>[2x]MHHHHHHQIGWRREGIKYRRNELFLDVLESVNLLMSPQGQVLSAHVSGRVVMKSYLSGMPECKFGMNDKIVIEKQGKGTADETSKSGKQSIAIDDCTFHQCVRLSKFDSERSISFIPPDGEFELMRYRTTKDIILPFRVIPLVREVGRTKLEVKVVIKSNFKPSLLAQKIEVRIPTPLNTSGVQVICMKGKAKYKASENAIVWKIKRMAGMKESQISAEIELLPTNDKKKWARPPISMNFEVPFAPSGLKVRYLKVFEPKLNYSDHDVIKWVRYIGRSGIYETRC;>SDLLAWDPLFG[2x]

Proper operation of the pivotal CME cargo adaptor AP2 requires membrane-localized Fer/Cip4 homology domain-only proteins (FCHO). The AP2 complex, composed of α, β2, μ2, and σ2 subunits, is pivotal to mammalian CCV formation, and its deletion is embryonically lethal in mice. FCHO1 and FCHO2 are similar in overall domain arrangement —folded N-terminal acidic phospholipid-binding homodimerization F-BAR domains and C-terminal folded μ-homology domains (μHD) separated by a ~300-residue, low-complexity intrinsically disordered protein linker, which has been suggested to participate in AP2 activation, although how it does so is undetermined. We dissect the network of interactions between the FCHO interdomain linker and AP2, which concentrates, orients, tethers, and partially destabilizes closed AP2 at the plasma membrane.

Crystals of a complex of Cμ2 and a peptide corresponding to this WxxL signal were grown, diffracted to 1.7-Å resolution, and were solved by MR using 1.9-Å unliganded Cμ2 as a search model. Binding was dependent on the presence of the tryptophan side chain as the homologous sequence from FCHO1, which does not contain a tryptophan, showed no binding. The mode favored will likely be context dependent, and it will likely be affected by multiple spatial and temporal factors in a nascent CCP including how many other α-appendage binding CCV proteins are present and whether the YxxΦ site of Cμ2 is accessible and/or occupied by cargo. These binding modes are likely to be in dynamic equilibrium with each other. The absence of WxxL in the C block of neuronally enriched FCHO1 but its presence in the ubiquitously expressed FCHO2 may reflect the paucity of YxxΦ-containing cargo found in synaptic CCVs that could compete out WxxL from Cμ2, which, if it did not occur, could slow or stall CCV formation. Thus, C blocks of all muniscin family members can bind to the α-appendage platform in a manner that is competitive with the binding of FxDxF and DP[FW] motifs of accessory CME proteins, and in addition, the partially overlapping WxxL sequence found only in FCHO2 can bind to the Cμ2 YxxΦ cargo–binding site and therefore potentially stabilize the unclosed but not-yet-open form of AP2.> MSILHTVNKSPFERNSLESCLKFATEGASVLLFEDGIYAALAGTRVESQVTEALGKLKLYV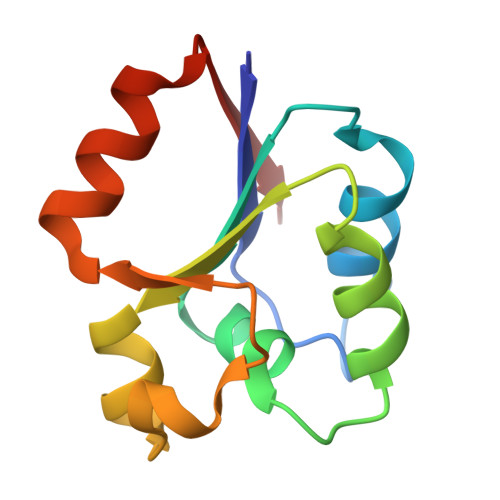LGPDLKARGFSDERVIPGISVVDYAGFVDLTTECDTVQAWL>[11x]QAATCNHTVMALMAS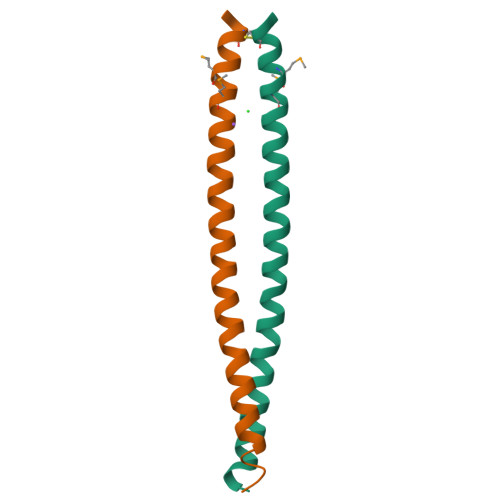LDAEKAQGQKKVEELEGEITTLNHKLQDASAEVERLRRENQVLSVR> MDELVKALERAGYLLTPSAYYLLVDHFKEGKFSLVELVKFAKSKGVFIIDGDLAYEFLQFLGLGVPQEIKESYISTGEEAEKTVESQETRASELEEGGVSQVSSGELQELKEESPEISTTEEEIGGLELVQSSISTGSEVEYNNGENGESVVVLDKYGYPILYAPEEIGEEKEYSKYEDVVIEWNPSVTPVQIEKNYEVKFDVRQVKLRPPKVKNGSGKEGEIIVEAYASLFKSRLSKLKRILRENPEISNVVDIGKLNYVSGDEEVTIIGLVNSKRETNRGLIFEVEDKTGIVKVFLPKDSEDYREAFKVLPDAVVAFKGFYSKKGIFFANKFYLPDVPLYRKQKPPLEEKVYAILISDIHVGSREFCEKAFLKFLEWLNGHVESKEEEEIVSRVKYLIIAGDVVDGIGIYPGQYSDLVIPDIFDQYEALANLLANVPEHITMFIGPGNADAARPAIPQPEFYKEYAKPIYKLKNAIIISNPAVIRLHGRDFLIAHGRGIEDVVSFVPGLTHHKPGLPMVELLKMRHLAPTFGGKVPIAPDPEDLLVIEEVPDLVQMGHVHVYDAVVYRGVQLVNSATWQAQTEFQKMVNIVPTPAKVPVVDVESARVVKVLDFSGWC;> GTGDGSELPKEMEEYFEMLQREIDKAYEIAKKARAQGKDPSLDVEIPQATDMAGRVESLVGPPGVAKRIRELVKEYGKEIAALKIVDEIIEGKFGDLGSREKYAEQAVRTALAILTEGIVSAPIEGIANVKIKRNTWADNSEYLALYYAGPIRSSGGTAQALSVLVGDYVRRKLGLDRFKPSEKHIERMVEEVDLYHRAVTRLQYHPSPEEVRLAMRNIPIEITGEATDDVEVSHRDVPGVETNQLRGGAILVLAEGVLQKAKKLVKYIDKMGIEGWEWLKEFVEAKEKGEPKEEGKEESLAESTLEETKVEVDMGFYYSLYQKFKEEIAPSDKYAKEVIGGRPLFSDPSKPGGFRLRYGRSRASGFATWGINPATMILVDEFLAIGTQLKTERPGKGAVVTPVTTIEGPIVKLKDGSVLRVDDYNLALKVREDVEEILYLGDAVIAFGDFVENNQTLLPANYCEEWWILEFVKALKEIYEVHLEPFTENEEESIEEASDYLEIDPEFLKEMLRDPLRVKPPVELAIHFSEVLGIPLHPYYTLYWNSVEPKDVEKLWRLLKNYAEIEWSNFRGIKFAKKIVISQEKLGDSKRTLELLGLPHTVRDGNVIVDYPWAAALLTPLGNLNWEFMAKPLYATIDIINENNEIKLRDRGISWIGARMGRPEKAKERKMKPPVQVLFPIGLAGGSSRDIKKAAEEGKVAEVEIAFFKCPKCGHVGPEHLCPNCGTRKELLWVCPRCNAEYPESQAEGYNYTCPKCNVKLRPYAKRKIRPSELLNRAMENVKVYGVDKLKGVMGMTSGWKMPEPLEKGLLRAKNDVYVFKDGTIRFDATDAPITHFRPREIGVSVEKLRELGYTHDFEGKPLVSEDQIVELKPQDIILSKEAGRYLLKVAKFVDDLLEKFYGLPRFYNAEKMEDLIGHLVIGLAPHTSAGIVGRIIGFVDALVGYAHPYFHAAKRRNCDGDEDAVMLLLDALLNFSRYYLPEKRGGKMDAPLVITTRLDPREVDSEVHNMDIVRYYPLEFYEATYELKSPKELVGVIERVEDRLGKPEMYYGLKFTHDTDDIALGPKMSLYKQLGDMEEKVRRQLEVAKRIRAVDEHGVAEKILNSHLIPDLRGNLRSFTRQEFRCVKCNTKFRRPPLNGKCPVCGGKIVLTVSKGAIEKYLGTAKMLVTEYNVKNYTRQRICLTERDIDSLFENVFPETQLTLIVNPNDICQRLVMARTGEVNKSGLLENLSNGSKKTEKAEKAEKPRKKSDEKPKKKRVISLEEFFSRKSK;>MRGSHHHHHHGSMPFEIVFEGAKEFAQLIETASRLIDEAAFKVTEEGISMRAMDPSRVVLIDLNLPASIFSKYEVDGEETIGVNMDHLKKVLKRGKAKETLILRKGEENFLEISLQGTATRTFKLPLIDVEEIEVDLPELPFTAKVVILGDVIKEAVKDASLVSDSMKFIAKENEFTMRAEGETQEVEVKLTLEDEGLLDIEVQEETKSAYGISYLSDMVKGLGKADEVTIKFGNEMPMQMEYYIRDEGRLIFLLAPRVEE[3x]

The bacterial sliding clamp is referred to as the β clamp, whereas the eukaryotic and archaeal sliding clamp protein is called the proliferative cell nuclear antigen (PCNA). Clamps are constructed from either two (β) or three monomers (PCNA) to yield a ring composed of six domains, which share similar protein folds. Hence, across every domain of life, the extraordinary efficacy of the replicative polymerase complex is dependent on their interaction with sliding clamps, which encircle DNA and greatly enhance their processivity. We have shown that PolD uses two distinct PIP-boxes for molecular recognition of PCNA, which are located in the C-terminal region of their DP2 subunit.

Here we present the cryo-EM structure of the DNA-bound PolD–PCNA complex from Pyrococcus abyssi at 3.77 Å using an integrative structural biology approach, combining cryo-EM, X-ray crystallography, protein–protein interaction measurements, and activity assays. A defining feature of the PolD–PCNA–DNA ternary complex is its compactness: the radius of the PCNA ring and the clamp-like PolD DNA-binding domain match perfectly. Interaction with PCNA nearly doubles the positively charged surface formed by the PolD active site, making a 60 Å-long DNA-binding site. This structure thus rationalizes how PCNA enhances the processivity of PolD: interaction with PCNA perpetuates the interactions with the nascent DNA duplex when it exits the PolD clamp, thereby preventing the polymerase from falling off prematurely. Although the DNA bound by the PolD–PCNA complex is predominantly in the B-form, interaction with the PolD clamp causes a distortion of the DNA region located next to the active site. Although PolD extensively interacts with the nascent DNA duplex, the PCNA channel exposes several positively charged residues, which are pointed towards the DNA backbone and make labile transient polar contacts with DNA. The cryo-EM map shows how PCNA is tethered to PolD through multiple contacts that involve both clamp-1 and clamp-2 domains of DP2. First, the α-helices, α-40, and α-41 of the clamp-1 domain are connected by a loop of 17 amino acids, which is hooked into PCNA. This loop binds to the canonical PCNA PIP-binding pocket through an internal PIP-box (iPIP), which has never been identified so far. Strikingly, both cPIP and the linker are not visible in the cryo-EM density of the DNA-bound PolD–PCNA complex.>MFKSFFPKPGTFFLSAFVWALIAVIFWQAGGGDWVARITGASGQIPISAARFWSLDFLIFYAYYIVCVGLFALFWFIYSPHRWQYWSILGTALIIFVTWFLVEVGVAVNAWYAPFYDLIQTALSSPHKVTIEQFYREVGVFLGIALIAVVISVLNNFFVSHYVFRWRTAMNEYYMANWQQLRHIEGAAQRVQEDTMRFASTLENMGVSFINAIMTLIAFLPVLVTLSAHVPELPIIGHIPYGLVIAAIVWSLMGTGLLAVVGIKLPGLEFKNQRVEAAYRKELVYGEDDATRATPPTVRELFSAVRKNYFRLYFHYMYFNIARILYLQVDNVFGLFLLFPSIVAGTITLGLMTQITNVFGQVRGAFQYLINSWTTLVELMSIYKRLRSFEHELDGDKI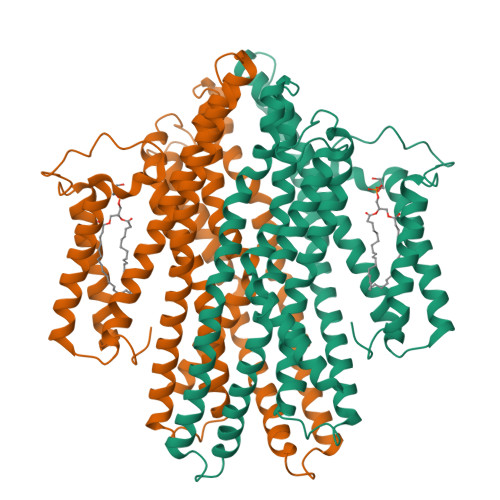QEVTHTLS[2x]>GQPPRRYTPDWPSLDSRPLPAWFDEAKFGVFIHWGVFSVPAWGSEWFWWHWQGEGRPQYQRFMRDNYPPGFSYADFGPQFTARFFHPEEWADLFQAAGAKYVVLTTKHHEGFTNWPSPVSWNWNSKDVGPHRDLVGELGTALRKRNIRYGLYHSLLEWFHPLYLLDKKNGFKTQHFVSAKTMPELYDLVNSYKPDLIWSDGEWECPDTYWNSTNFLSWLYNDSPVKDEVVVNDRWGQNCSCHHGGYYNCEDKFKPQSLPDHKWEMCTSIDKFSWGYRRDMALSDVTEESEIISELVQTVSLGGNYLLNIGPTKDGLIVPIFQERLLAVGKWLSINGEAIYASKPWRVQWEKNTTSVWYTSKGSAVYAIFLHWPENGVLNLESPITTSTTKITM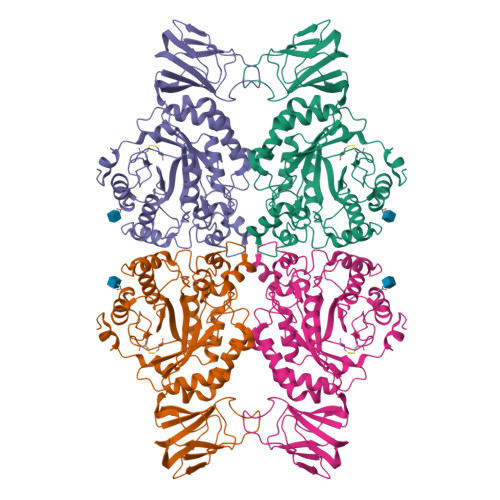LGIQGDLKWSTDPDKGLFISLPQLPPSAVPAEFAWTIKLTGVK[4x]>KETAAAKFERQHMDSSTSAASSSNYCNQMMKSRNLTKDRCKPVNTFVHESLADVKAVCSQKKVTCKNGQTNCYQSKSTMRITDCRETGSSKYPNCAYKTTQANKHI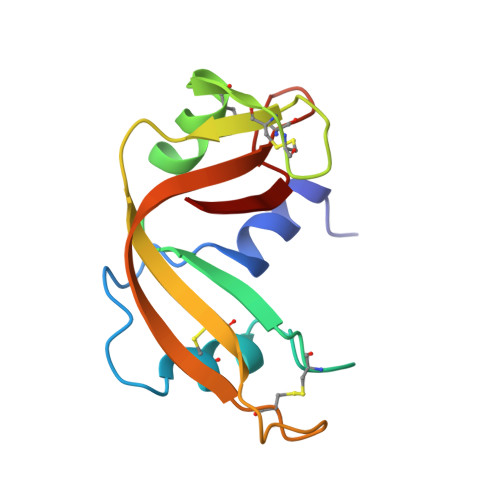IVACGGKPYVPVHFDASV[2x]> 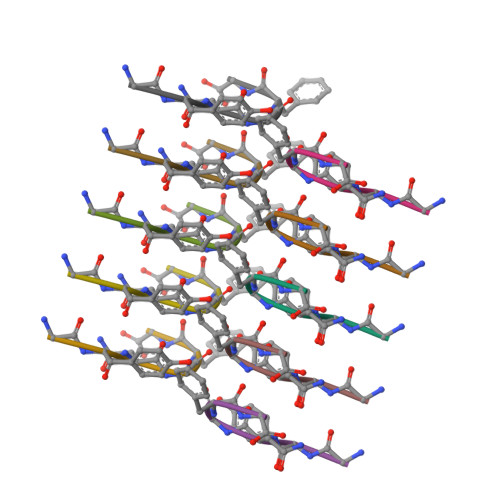GYNGFG> PCCDHCSCTKSIPPQCRCTDLRLDSCHSACKSCICTLSIPAQCVCDDIDDFCYEP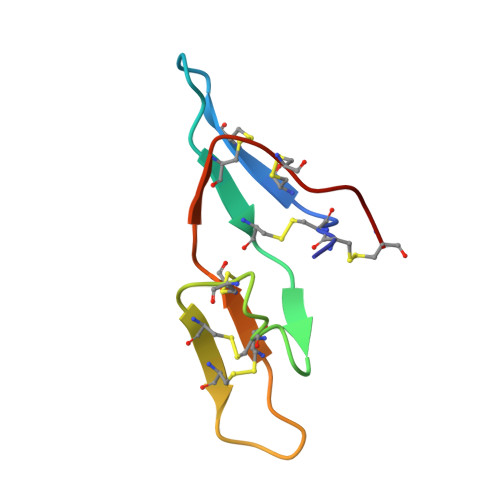C>MASMTGGQQMGRGSSTSLYKKAGLMPSPMEDIEEILITEEQLKAKVKELGEMITRDYEGKDLVLIGVLKGAIMFMSGLSRAIDLPLSIDFLAVSSYGSSTKSS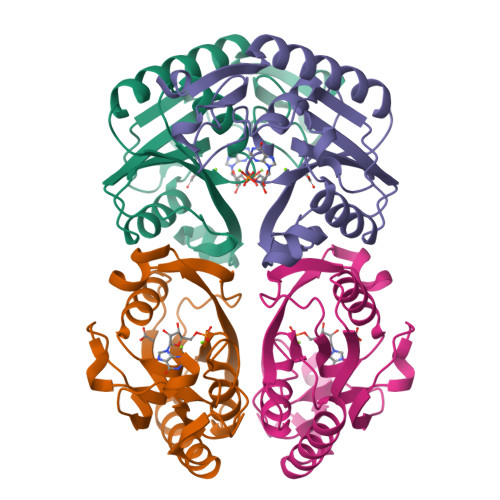GIVKIIKDHDIDIEGKDVLIVEDIIDSGLTLAYLRETLLGRKPRSLKICTILDKPERREADVKVDYCGFKIPDKFVVGYGLDYAEKYRNLPFIGVLKPELYK[2x]1-desthiobiotinylpyrene | C26 H26 N2 O2 | 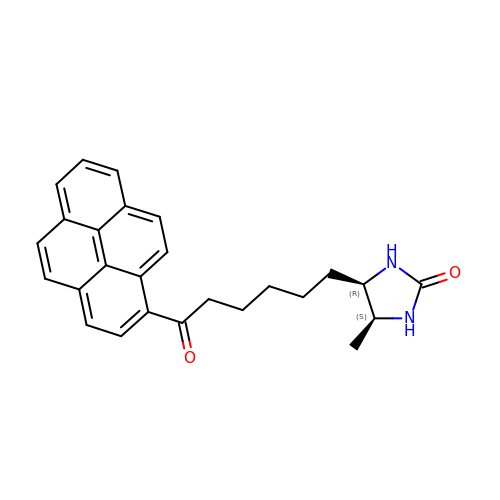GEJQOLRONNVYHQ-KSFYIVLOSA-N> GSHMASMTGGQQMGRGSTLSEYVQDFLNHLTEQPGSFETEIEQFAETLNGCVTTDDALQELVELIYQQATSIPNFSYMGARLCNYLSHHLTISP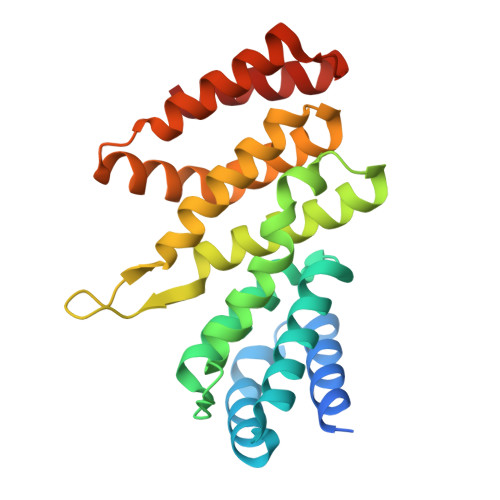QSGNFRQLLLQRCRTEYEVKDQAAKGDEVTRKRFHAFVLFLGELYLNLEIKGTNGQVTRADILQVGLRELLNALFSNPMDDNLICAVKLLKLTGSVLEDAWKEKGKMDMEEIIQRIENVVLDANCSRDVKQMLLKLVELRSS> GSLRGTTQKVNRIREITAMKTVEALQISAQLTQLHEVDMTRVAELRKKNKPAFIEKHGVNLTYLPFFVKAVVEALVSHPNVNASFNAKTKEMTYHSSVNLSIAVDT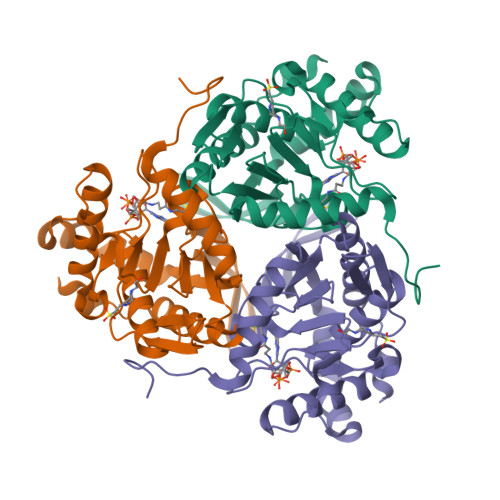PAGLLTPVIHDAQDLSIPEIAKAIVDLADRSRNNKLKPNDLSGGTFTITNIGSEGALSDTPILVPPQAGILGTGAIVKRPVVITEDGIDSIAIRQMVFLPLTYDHQVVDGADAGRFLTTIKDRLETANFEGDLQL> HHHHHHMPLDPRVEQFLAQMPPLNREGLSLAEARQQFKQGALLLDQMVPP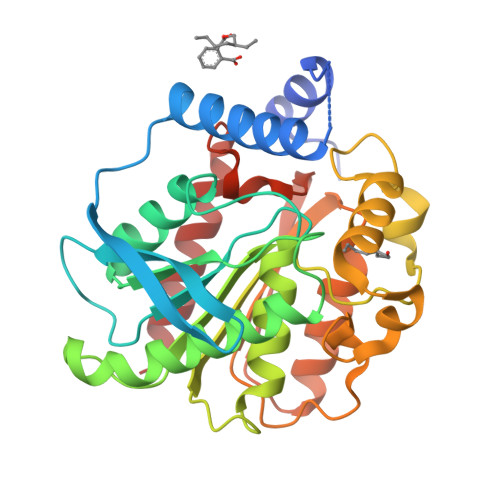PPVDTEDGTVVTTHGPVRIRRYIPDRLRFSHPLVFYHGGGFVFGDIDTHHGLVARLCQTVGATVISVDYSLAPEAKFPVPVAECIDVARWAAHEAPGWGLKPSIVVAGDSAGGNLAAVVSQRAKDESLPIAAQLLFYPALDMVHETPSKRDFARGYLLEADAMQWFGEQYLRTPDDVSHPWASPALSPDLTGLPPALVITAEYDPLRDEGEAYAEALRAAGVPTEQIRFDGMIHGFMTMPIFPQMEAAIEAVARFLERID> SHPALTQLRALRYSKEIPALDPQLLDW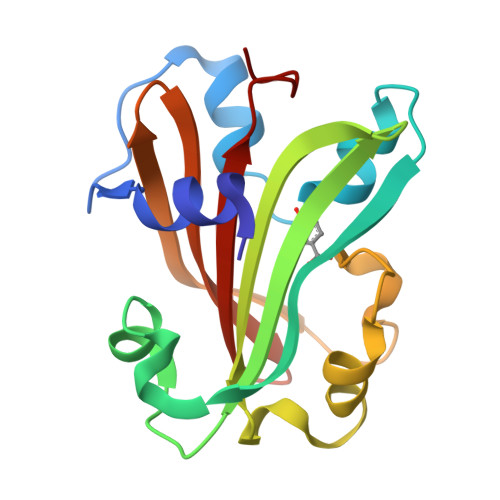LLLEDSMTKRFEQQGKTVSVTMIREGFVEQNEIPEELPLLPKESRYWLREILLCADGEPWLAGRTVVPVSTLSGPELALQKLGKTPLGRYLFTSSTLTRDFIEIGRDAGLWGRRSRLRLSGKPLLLTELFLPASPLY>[2x]MSNKYRVRKNVLHLTDTEKRDFVRTVLILKEKGIYDRYIAWHGAAGKFHTPPGSDRNAAHMSSAFLPWHREYLLRFERDLQSINPEVTLPYWEWETDAQMQDPSQSQIWSADFMGGNGNPIKDFIVDTGPFAAGRWTTIDEQGNPSGGLK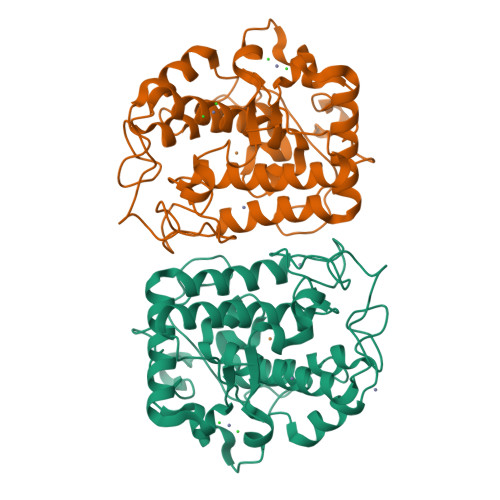RNFGATKEAPTLPTRDDVLNALKITQYDTPPWDMTSQNSFRNQLEGFINGPQLHNRVHRWVGGQMGVVPTAPNDPVFFLHHANVDRIWAVWQIIHRNQNYQPMKNGPFGQNFRDPMYPWNTTPEDVMNHRKLGYVYDIELRKSKRSSHHHHHH> TFPTYKCPETFD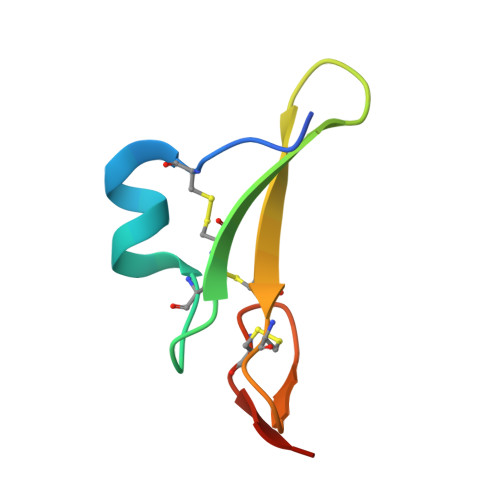AWYCLNDAHCFAVKIADLPVYSCECAIGFMGQRCEYKEID>[12x]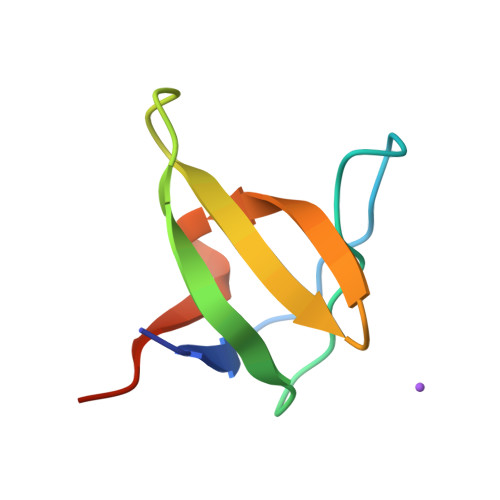MVDYIVEYDYDAVHDDELTIRVGEIIRNVKKLQEEGWLEGELNGRRGMFPDNFVKEIKRETE> GSPPARKEKTKVKESVSRVEKAKQKSAQQELKQRQRAEIYALN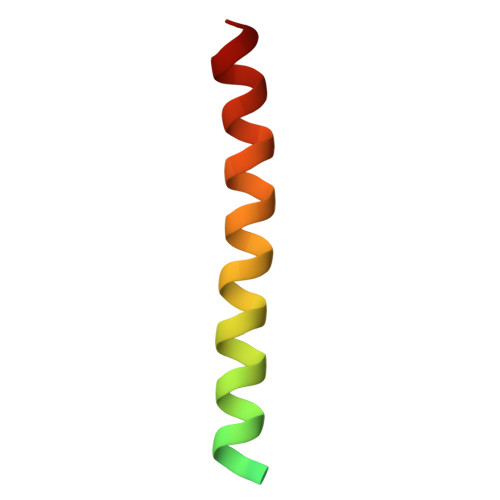RVMTEL> GSTPTINIPASPFMQKLGFGTGVNVYLMKRSPRGLSHSPWAVKKINPICNDHYRSVYQKRLMDEAKILKSLHHPNIVGYRAFTEANDGSLCLAMEYGGEKSLNDLIEERYKASQDPFPAAIILKVALNMARGLKYLHQEKKLLHGDIKSSNVVIKGDFETIKICDVGVSLPLDENMEVTDPEACYIGTEPWKPKEAVEENGVITDKADIFAF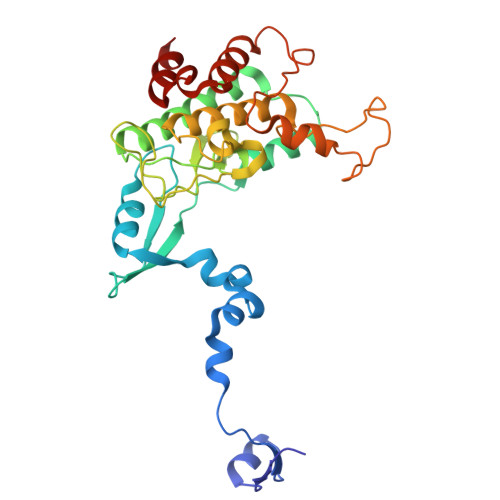GLTLWEMMTLSIPHINLSNDDDDEDKTFDESDFDDEAYYAALGTRPPINMEELDESYQKVIELFSVCTNEDPKDRPSAAHIVEALETA>HHHHHHGSPSRSAEIMKHGYPGFTNVRTYEDFVLSYDYKTRTAHWVCEHLTPERLKHAEGVDRKLCEFKPDITFPQKFLSQNTDYKCSGFDRGHLAAAGNHRKSQLAVDQTFYLSNMSPQVGRGFNRDKWNDLEMHCRRVAKKMINSYIITGPLYLPKLEGDGKKYIKYQVIGDNNVAVPTHFFKVALFEVTPGKFELESYILPNAVIEDTVEISKFHVPLDAVERSAGLEIFARLDPKS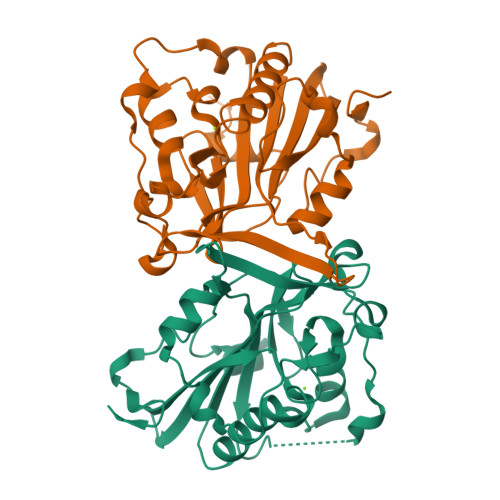IVKENGAKK[2x]> MHHHHHHMPIIEQVRAREILDSRGNPTVEVEVALIDGTFARAAVPSGASTGEHEAVELRDGGDRYGGKGVQKAVQAVLDEIGPAVIGLNADDQRLVDQALVDLDGTPDKSRLGGNAILGVSLAVAKAAADSAELPLFRYVGGPNAHILPVPMMNILNGGAHADTAVDIQEFMVAPIGAPSFVEALRWGAEVYHALKSVLKKEGLSTGLGDAGGFAPDVAGTTAALDLISRAIESAGLRPGADVALALDAAATEFFTDGTGYVFEGTTRTADQMTEFYAGLLGAYPLVSIEDPLSEDDWDGWAALTASIGDRVQIVGDDIFVTNPERLEEGIERGVANALLVKVNQIGTLTETLDAVTLAHHGGYRTMISHRSGETEDTMIADLAVAIGSGQIKTGAPARSERVAKYNQLLRIEEALGDAA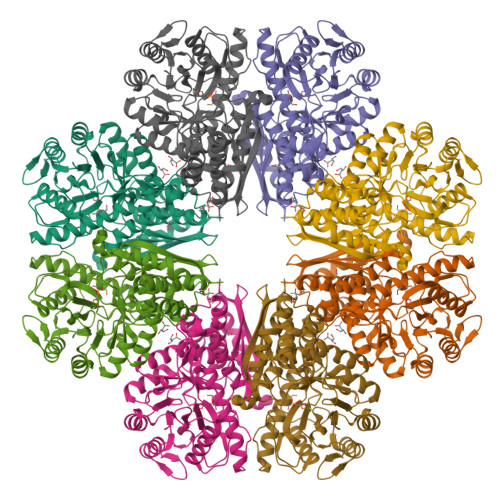RYAGDLAFPRFACETK> SGALQRAVREIPWKSRQDILRERERPVYAAECRGTPRREYSKNVIDGVRVKPTFNPFVKLNKAKRYVLDNWPSRNWDDWSPYRCYVRG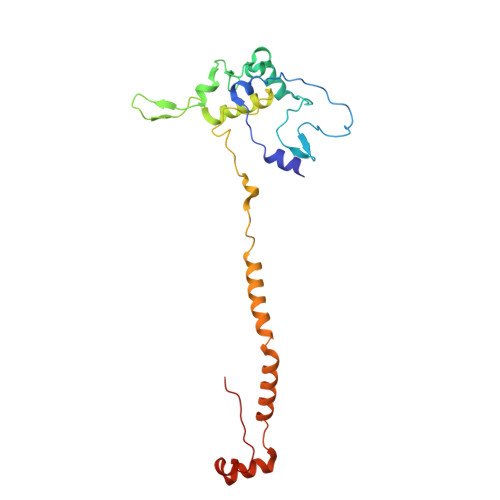SRRRYNIPQDLLPYKDELGEWHPPRLSARYQADVKKQYLMNNLPWVWQKDFYEGKMHFGDREPLGPKVWYRKAFREERVKEAMRKMDDLVLDYRQENRDRRRYNWFEKVVHDFAGEEIATQFIRKRKEPKL>SNAMKKVQGIYRAPR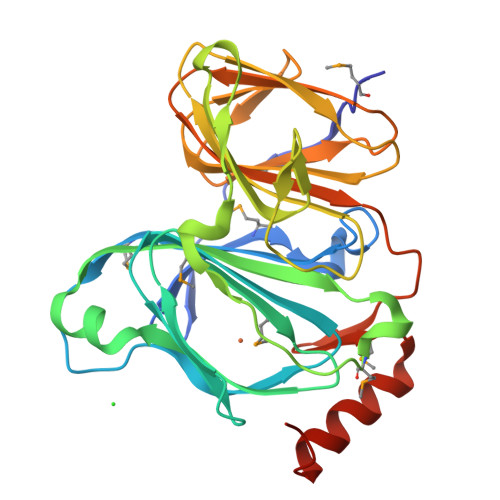QHWVGDGFPVRSMFSYQSHGKQLSPFLLLDYAGPMDFTPTTQRRGVGQHPHRGFETVTIVYHGEVEHRDSTGNGGIIGPGDVQWMTAGAGILHEEFHSDAFAQKGGPFEMVQLWVNLPAKDKMTAPGYQAIRREAIPQVNLPDDAGNLRVIAGEYAGNIGPAKTFSPLNVWDIRLTQGKSCEFSLPAGWNTALIVLHGTLLVNGDAIAREAEMVLLDPTGTHLSIEANNDTVLLLLSGEPIDEPIVGYGPFVMNTQAQIAEAIADFNGGRFGNMDVA[2x]>SPSTNRKYPPLPVDKLEEEINRRMADDNKLFREEFNALPACPIQATCEAASKEENKEKNRYVNILPYDHSRVHLTPVEGVPDSDYINASFINGYQEKNKFIAAQGPKEETVNDFWRMIWEQNTATIVMVTNLKERKECKCAQYWPDQGCWTYGNVRVSVEDVTVLVDYTVRKFCIQQVGDVTNRKPQRLITQFHFTSWPDFGVPFTPIGMLKFLKKVKACNPQYAGAIVVHCSAGVGRTGTFVVIDAMLDMMHSERKVDVYGFVSRIRAQRCQMVQTDMQYVFIYQ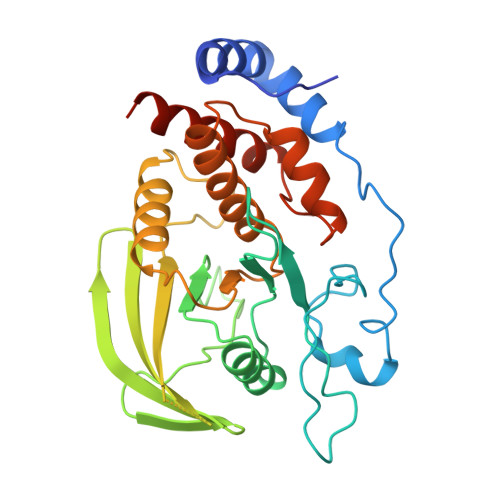ALLEHYLYGDTELEVT[2x]[(3R)-3-{[(4M)-4-(4-cyclopropyl-2-phenyl-1H-imidazol-1-yl)pyrimidin-2-yl]amino}pyrrolidin-1-yl](1,3-thiazol-2-yl)methanone 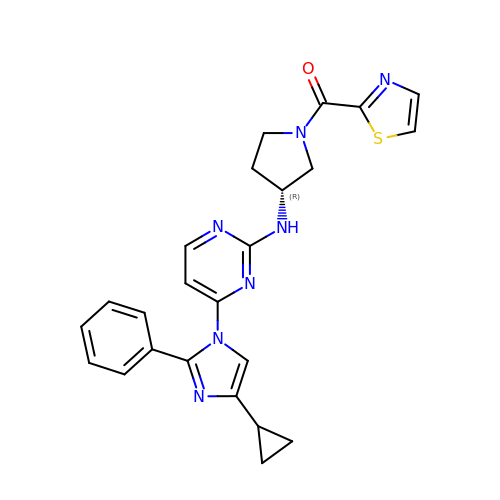| C24 H23 N7 O S | WMOACOPVFVMARL-GOSISDBHSA-N> MFIINSDFHRGNMEQYQKAQKLSFDPAELLRTSLNVGDIVLLKQCTSELTMCVNLPQSTTDPRYTFAKKDGTLVYAMKNSVILRIPKDLPEEVNQLLKRESNHPYQKIGTIKNSSNETEILPVLTRQLIVSFTLATFTKFAWTQLPIVLKKLELIHRYLQDSRGSKHVNFMSLVRIIKNLNIKEATDAINGDAYVRKVIDESMSVVNKSIDPTTLLATYWGVREQQQNNLWGSVYTNTALLSPTTVAVLPLKKAHLFYQEVITRLESNDYQEIKAFAKLVNDKDYHSIAKRYDYIRTLLNDYAAGNIEENAVLTTIISKIFRHIDMYRDQDVTRSLCGKLLVEISPQSNSSNFILGNWDLNIPKSSGISSVEQKLYDTAMPTIVSDTDRYDFGDMPVFCIDSEDAHEINDGISIEELDGVRSRIHIHIADPAGLFPESFDYTKSGISDDVLRVSLKRAFTTYLPDLVVPMLPKSFCNRADLGKHDRKTETISFSFELVNKEDGGLHVDYDTFQVRLGIVSNFPKVTYDKVDSILNGDDNSLPSKQKKQLELLHTLATKLLHKRIHDDNAVVFGDGFNKGLVSLSPDDDGELCIPTFYDQSQTKSTLLVSEFMILTNKLCAAFFQENKIPGVYRCYNGLNLGNQAKAQFELLKENIKLGKLPSLKDITKISSQLSSSFYSPFPLPHKMIGNTAYLTVTSPMRRGPDLINHLQLHRFLKKLPLCFKQEYLDQYVWSFQARADILKIFQRHSSTYWTLKHLEQSGTKTHDVIVTSVPQNGTVNCLFPEYSYARGTLKLDPAMKKIPRIGDTIRHCKVESIHPLDGILTLTHVNRK;> MIYTTDKEFKKNLENALAHVYSTQIENSAPDQVEFRKVAWLRLKDMLYNQLLDKNLPAKINGYDPGLMETISPTQPQHIIPHLVKMNKIDQLIWKKITGKTEGVTKYEQFQYLLSSYYDCILNQEIIPSMLNTGTDDSVHSVDFSNPAEWFPEARKIRRHIIMHVGPTNSGKTFRSLQKLKAADRGYYAGPLRLLAREVYEKFKHENVRCNLLTGEEVIKDLDEMGNEANLTSGTIEMIPLNQNFDVVVLDEIQMMADLDRGWAWTNALLGAKAKEVHCCGEASTIPLIKKIVEMTGDKLTINEYERMGKLVVEEEALTKGYHSLKKGDCVVAFSKKAILDLKLEIEKKTELKAAVIYGSLPPETRVKQANLFNSGEFDILIASDAIGMGLNLSIDRVVFTTSKKFDGRDMVDMTSSAIKQIGGRAGRFKQNIHDNGELPVGYITAVKPNVLKAVREAINAPIEYLTSATTWPTDEICTHVMTRFMPGTTCKTLLETIAADIEQSSNKLFQICDLKARMSAIEIIDSMEDITFSDKLRLSNAPLKDFPLVKAAFKKFCDTIARGHTRGLLSYRFPFDILNLKYIYTEKHGLEEYEALYNIIMLFFWLSNRYPNYFIDQESASELKNFCEMIIFEKIDHLKRNPY

The mtEXO complex is composed of two subunits: the nucleotide triphosphate (NTP)-dependent RNA helicase Suv3 and the 3′-to-5′ exoribonuclease Dss13. Dss1 individually has low RNase activity, and the robust nucleolytic activity of the entire degradosome complex nearly completely depends on ATP, an unprecedented feature that is not found in other known RNA-degrading systems. To understand the structure and mechanism of the yeast mitochondrial RNA degradosome, we present crystal structures of Dss1 nuclease and the mtEXO complex of the yeast Candida glabrata (Cg). Our structural analysis revealed the architecture of the Cg-mtEXO complex, in which the helicase motor feeds the 3′ end of the RNA into the catalytic channel of Dss1 for efficient and processive degradation.

We obtained crystals for Dss170–900 D477N in complex with Suv343–685 in the presence of a dsRNA substrate with a 3′ 8 nt overhang (annealed 20Tx and 12Bx oligonucleotides) and ATP/Mg2+. The final model was refined at 3.55 Å resolution. The structures of Cg-Dss1 alone and in the Cg-mtEXO complex are very similar (RMSD of 0.77 Å over 533 C-α atoms); therefore, Dss1 does not change its conformation upon interactions with Suv3. In the Cg-mtEXO structure, Suv3 is positioned close to the small accessory domains of Dss1: β-barrel, HTH, WH, and S1 which decorate the catalytic RNB domain and form a funnel around the entry to the RNA-binding channel. Two main interfaces are formed between Cg-Suv3 and the small domains. The first and much more extensive interface involves the HTH domain of Cg-Dss1 (residues Tyr338, Thr383, Ser386, Arg390, Asp397, and Val400) and residues from the B-α-1′ helix of the first RecA domain of Cg-Suv3 and its vicinity (Asn187, Glu190, Lys197, and Arg199). The second smaller Suv3-Dss1 interface forms between the C-terminal domain of the Cg-Suv3 helicase and a long kinked α-helix of the WH domain of Cg-Dss1. This interaction involves hydrophobic patches that comprise residues Trp210 and Leu213 of Cg-Dss1 and Met523 and Phe574 of Cg-Suv3. Compared with human SUV3, this domain of Cg-Suv3 in the mtEXO complex has a different position relative to the rest of the structure. It is rotated by ~90° around a hinge between residues 172 and 185 and interacts with a cleft between the WH and HTH domains and RNB domain of Cg-Dss1. A 6 nt RNA fragment is present in the Cg-mtEXO structure inside the RNA-binding channel of Dss1 and it is superimposable with the RNA observed in Cg-Dss1 forming the same contacts with the protein.> KSSKISEQLKCCSGILKEMFAKKHAAYAWPFYKPVDVEALGLHDYCDIIKHPMDMSTIKSKLESREYR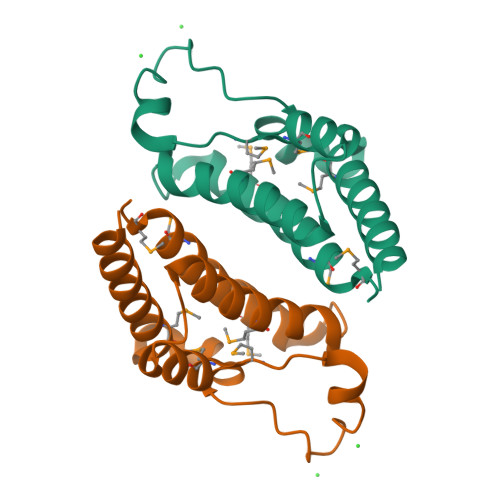DAQEFGADVRLMFSNCYKYNPPDHEVVAMARKLQDVFEMRFAKMPD>[2x]MMLSLNNLQNIIYNPVIPFVGTIPDQLDPGTLIVIRGHVPSDADRFQVDLQNGSSMKPRADVAFHFNPRFKRAGCIVCNTLINEKWGREEITYDTPFKREKSFEIVIMVLKDKFQVAVNGKHTLLYGHRIGPEKIDTLGIYGKVNIHSIGFSFSSHMRLPFAARLNTPMGPGRTVVVKGEVNANAKSF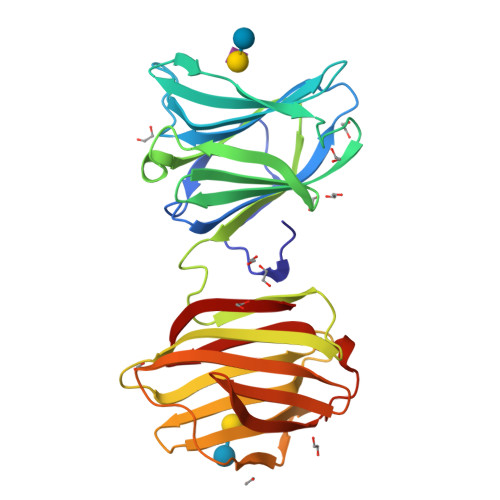NVDLLAGKSKDIALHLNPRLNIKAFVRNSFLQESWGEEERNITSFPFSPGMYFEMIIYCDVREFKVAVNGVHSLEYKHRFKELSSIDTLEINGDIHLLEVRSW> MVDQATLDKLEAGFKKLQEASDCKSLLKKHLTKDVFDSIKNKKTGMGATLLDVIQSGVENLDSGVGIYAPDAESYRTFGPLFDPIIDDYHGGFKLTDKHPPKQWGDINTLVGLDPAGQFIISTRVRCGRSLQGYPFNPCLTAEQYKEMEEKVSSTLSSMEDELKGTYYPLTGMSKATQQQLIDDHFLFKEGDRFLQTANACRYWPTGRGIFHNDAKTFLVWVNEEDHLRIISMQKGGDLKTVYKRLVTAVDNIESKLPFSHDDRFGFLTFCPTNLGTTMRAS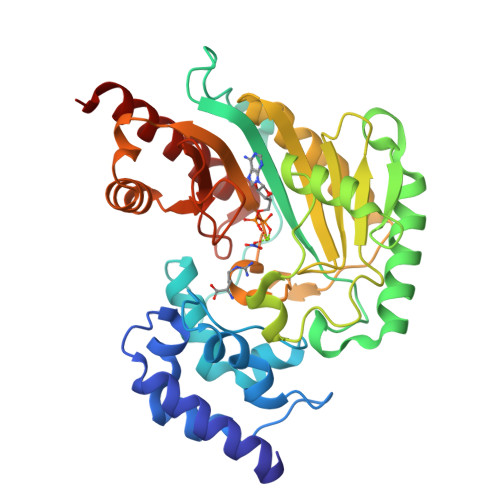VHIQLPKLAKDRKVLEDIASKFNLQVRGTRGEHTESEGGVYDISNKRRLGLTEYQAVREMQDGILEMIKMEKAAA>[2x]MSGASSSEQNNNSYETKTPNLRMSEKKCSWASYMTNSPTLIVMIGLPARGKTYVSKKLTRYLNWIGVPTKVFNLGVYRREAVKSYKSYDFFRHDNEEAMKIRKQCALVALEDVKAYLTEENGQIAVFDATNTTRERRDMILNFAEQNSFKVFFVESVCDDPDVIAANILEVKVSSPDYPERNRENVMEDFLKRIECYKVTYRPLDPDNYDKDLSFIKVINVGQRFLVNRVQDYIQSKIVYYLMNIHVQP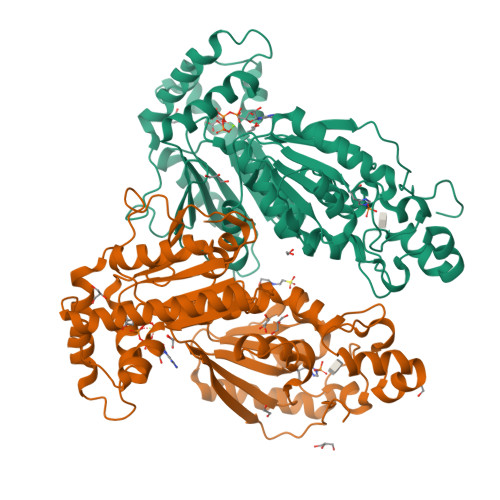RTIYLCRHGESEFNLLGKIGGDSGLSVRGKQFAQALRKFLEEQEITDLKVWTSQLKRTIQTAESLGVPYEQWKILNEIDAGVCEEMTYAEIEKRYPEEFALRDQEKYLYRYPGGESYQDLVQRLEPVIMELERQGNVLVISHQAVMRCLLAYFLDKGADELPYLRCPLHTIFKLTPVAYGCKVETIKLNVEAVNTHRDKPTNNFPKNQTPVRMRRNSFTPLSSSNTIRRPRNYSVGSRPLKPLSPLRAQDMQEGAD>[2x]GSHMNTLKKAFEILDFIVKNPGDVSVSEIAEKFNMSVSNAYKYMVVLEEKGFVLRKKDKRYVPGYKLIEYGSFVLRRFNIRDIAHDHLVDIMKRTGE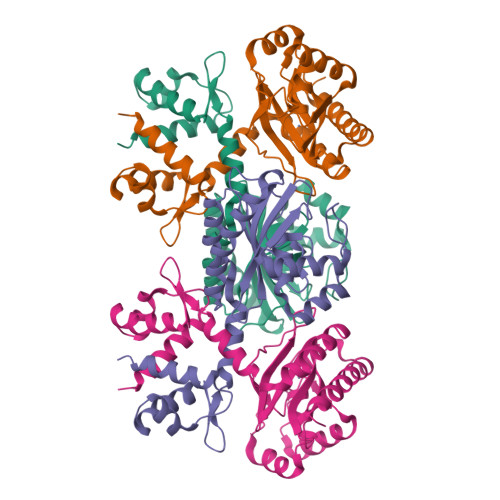TVHLILKDGFEGVYIDKVEGEQSIPMVSRLGMKVDLYSTASGKSILAFVPEKELKEYLKIVELKPKTPNTITNPRVLKRELEKIRKRGYAVDNEENEIGIMCVGVPIFDHNGYPVAGVSISGVARKFTEEKIEEYSDVLKEKAEEISRKLGY prop-2-en-1-yl (2S)-2-[(2S,3R)-3-(acetyloxy)-1-oxobutan-2-yl]-2,3-dihydro-1,3-thiazole-4-carboxylate | C13 H17 N O5 S | 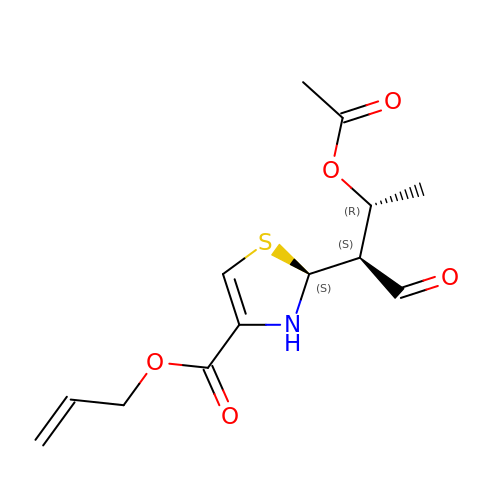KYVQFVHQVGHNFK-UISBYWKRSA-N> AHHHHHHVDDDDKMQTVGVHSIVQQLHR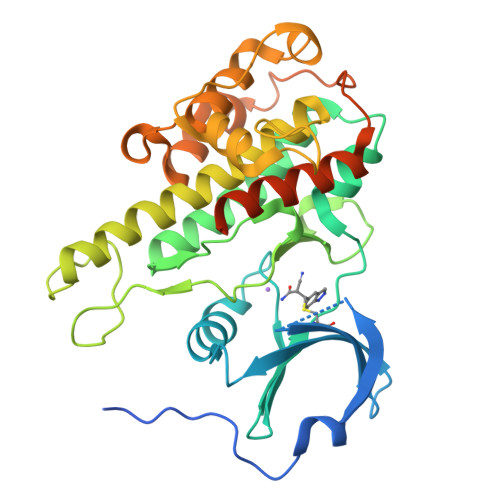NSIQFTDGYEVKEDIGVGSYSVCKRCIHKATNMEFAVKIIDKSKRDPTEEIEILLRYGQHPNIITLKDVYDDGKYVYVVTELMKGGELLDKILRQKFFSEREASAVLFTITKTVEYLHAQGVVHRDLKPSNILYVDESGNPESIRICDFGFAKQLRAENGLLMTPCYTANFVAPEVLERQGYDAACDIWSLGVLLYTMLTGYTPFANGPDDTPEEILARIGSGKFSLSGGYWNSVSDTAKDLVSKMLHVDPHQRLTAALVLRHPWIVHWDQLPQYQLNRQDAPHLVKGAMAATYSALNRNQSPVLEPVGRSTLAQRRGIKKITSTAL> SENQVTKVKDTNIFPYTGVVAFKSATGFVVGKNTILTNKHVSKNYKVGDRITAHPNSDKGNGGIY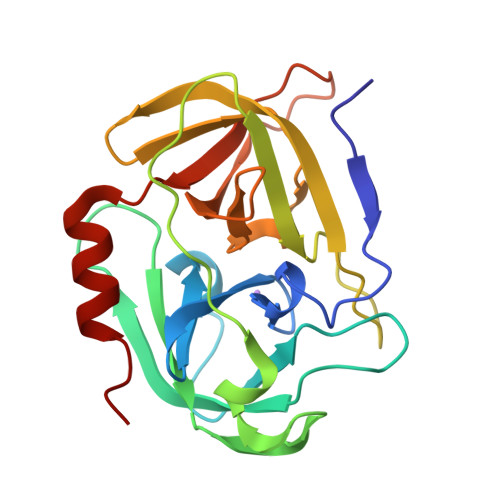SIKKIINYPGKEDVSVIQVEERAIERGPKGFNFNDNVTPFKYAAGAKAGERIKVIGYPHPYKNKYVLYESTGPVMSVEGSSIVYSAHTERGNSGSPVLNSNNELVGIHFASDVKNDDNRNAYGVYFTPEIKKFIAENIDKG>MYTMGLDIGSTASKGVILKNGEDIVASETISSGTGTTGPSRVLEKLYGKTGLAREDIKKVVVTGYGRMNYSDADKQISELSCHARGVNFII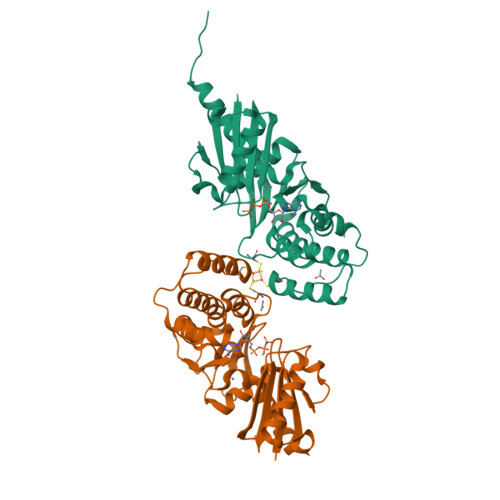PETRTIIDIGGQDAKVLKLDNNGRLLNFLMNDKCAAGTGRFLDVMAKIIEVDVSELGSISMNSQNEVSISSTCTVFAESEVISHLSENAKIEDIVAGIHTSVAKRVSSLVKRIGVQRNVVMVGGVARNSGIVRAMAREINTEIIVPDIPQLTGALGAALYAFDEAKESQKEVKNISAWSHPQFEK[2x]1-(2-hydroxyethyl)-3-methyl-6,7-dihydro-5~{H}-indazol-4-one 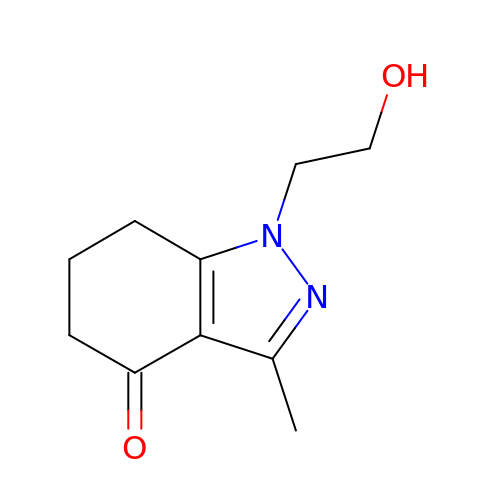| C10 H14 N2 O2 | NUFKJJIXCWBCHD-UHFFFAOYSA-N>GAHMKSTFKSEYPFEKRKAESERIADRFKNRIPVICEKAEKSDIPEIDKRKYLVPADLTVGQFVYVIRKRIMLPPEKA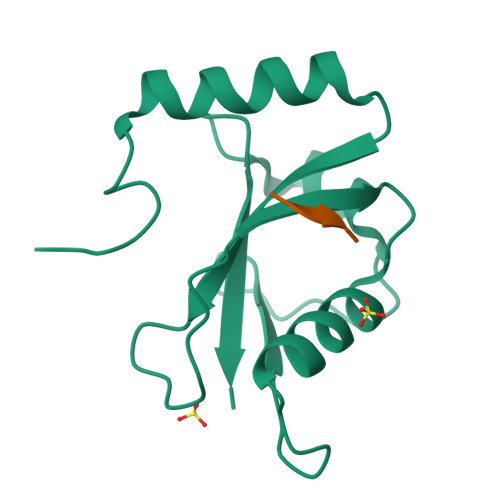IFIFVNDTLPPTAALMSAIYQEHKDKDGFLYVTYSGENTFG[4x];>WEEL[4x]Bacteriophage Casadabanvirus JBD30, from the order Caudoviricetes, is a temperate phage that infects the bacterium Pseudomonas aeruginosa. The virion of bacteriophage JBD30 is composed of an icosahedral capsid, long flexible non-contractile tail, and a baseplate. Using its baseplate, JBD30 attaches to Pseudomonas aeruginosa via the bacterial type IV pilus, whose subsequent retraction brings the phage to the bacterial cell surface.

The baseplate of JBD30 is terminated by a tripod formed by three trimers of receptor binding proteins (gp54). The receptor binding protein can be divided into thigh, knee, and foot domains. The N-terminal thigh domain (residues 1–118) connects the receptor binding protein to domain VII of the baseplate hub protein. The C-terminus of the baseplate hub protein docks into the centre of an α-helical bundle that each receptor binding protein contributes one α-helix to. The α-bundle is surrounded by peripheral β-sheets. The knee domain extends from the thigh domain, then bends back in an antiparallel β-sheet and ends in a short α-helix. The C-terminal foot domain of the receptor binding protein has the overall shape of a wedge, which is composed of a central β-sheet flanked by an α-helical spur. The JBD30 receptor binding protein foot domain is structurally similar to sugar-binding domains of hydrolytic enzymes (such as xylanase, glycoside hydrolase, endoglucanase, mannose, galactosidase) and an enzymatically active domain of bacteriophage cba120 tail spike protein. Aromatic residues of two adjacent foot domains form a hydrophobic cleft suitable for sugar binding. Therefore, we speculate that the foot domain of the JBD30 receptor binding protein recognizes and binds the host cell lipopolysaccharide O-antigen.

> MTLYMGPNTGLLINGLPGEGHYSDLIRMWRWDDFLRQPVVKGRVATLPTTGQAEGDTYIFTGSGSNQNRLARWWATGATTAIWEYMPPRLGWRVQVANETTPSGQVKTYEYSGTAWVELVGGMSDAPSDGKAYARESGAWTELGSAAKSALNVLPFMNLMPDMGRFAGTAANPLATMFTTSWTPSSFLNGWNGATVADGGKFAFDNSTNGGAGPALNARVQALLAAMGRTWTSVSRYGVEFFTAVLTAGSQTTTGSAGADGVTRYLCCSNGSKTVFNAGGWATVVMWLRVESGSAHISSAPYTTHRLWINGAVAAPGVVLPANQWVHLRFSMQSYNGYDNACPYIYASAGAQIAFACPAWFGGLVDPGIHVAPILTINGASA~{N}-methyl-2-(oxan-4-yloxy)-5-(2-oxidanylidene-2-phenylazanyl-ethoxy)benzamide | C21 H24 N2 O5 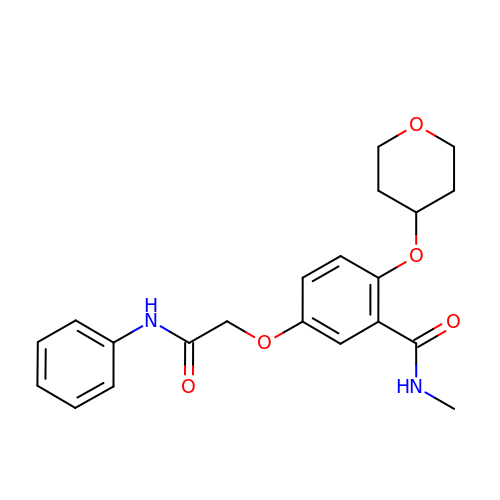| OLSMYKUQDJESEU-UHFFFAOYSA-N> MSDSFSLLSQITPHQRCSFYAQVIKTWYSDKNFTLYVTDYTENELFFPMSPYTSSSRWRGPFGRFSIRCILWDEHDFYCRNYIKEGDYVV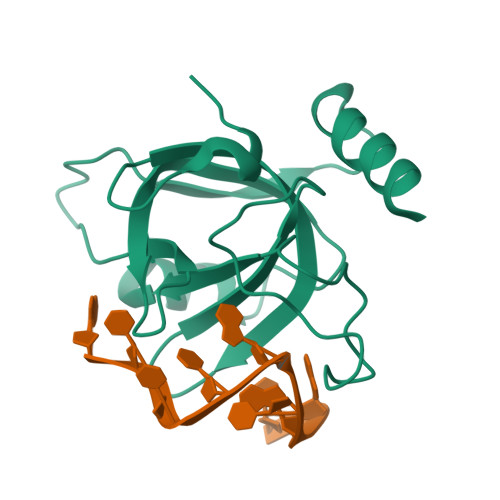MKNVRTKIDHLGYLECILHGDSAKRYNMSIEKVDSEEPELNEIKSRKRLYVQN benzene-1,2,3-tricarboxylic acid | C9 H6 O6 | 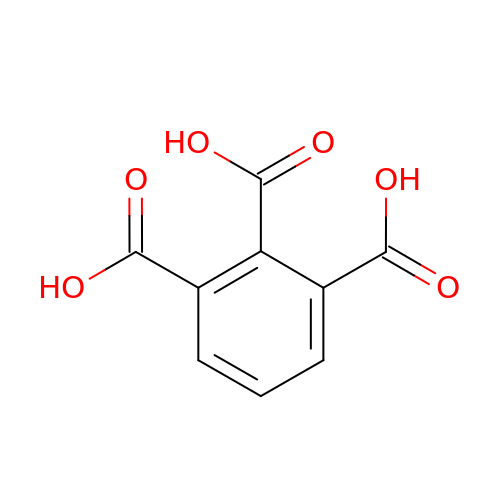UJMDYLWCYJJYMO-UHFFFAOYSA-N> DPEDLIDGIIFAANYLGSTQLLSDKTPSKNVRMMQAQEAVSRIKPEGESQPMTEVDLFISTQRIKVLNADTQEPMMDHPLRTISYIADIGNIVVLMARRRMPRSQYKMICHVFESEDAQLIAQSIG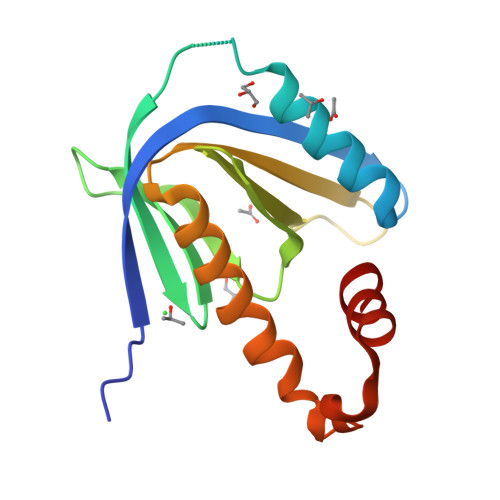QAFSVAYQEFLRANGINPEDLSQKEYSDLLNTQDMY> NEALCKKDGGVCSCNNNKNSVDCSSKKLTAIPSNIPADTKKLDLQSNKLSSLPSKAFHRLTKLRLLYLNDNKLQTLPAGIFKELKNLETLWVTDNKLQALPIGVFDQLVNLAELRLDRNQLKSLPPRVFDSLTKLTYLSLGYNELQSLPKGVFDKLTSLKELRLYNNQLKRVPEGAFD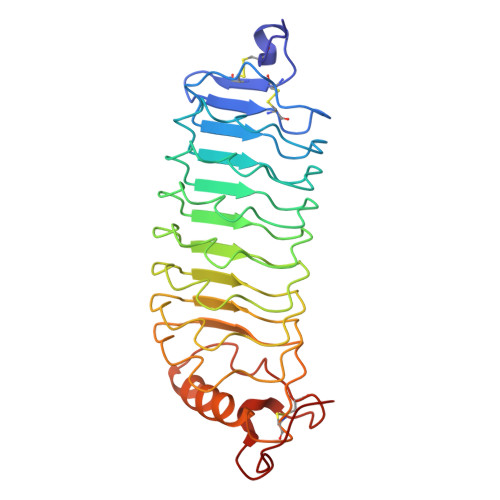KLTELKTLKLDNNQLKRVPEGAFDSLEKLKMLQLQENPWDCTCNGIIYMAKWLKKKADEGLGGVDTAGCEKGGKAVLEITEKDAASDCVSPN>GCAGCAGC[2x]

We have analyzed crystal structures of RNA containing CAG repeats in complex with synthetic cyclic mismatch-binding ligands (CMBLs). In total, three X-ray structures consisting of (GCAGCAGC)2-CMBL3a, one structure of (GCAGCAGC)2-CMBL3b and one (GCAGCAGC)2-CMBL4 complex have been analyzed. The models show well-defined interactions between the molecules in which the CMBLs mimic nucleobases as they form pseudo-canonical base pairs with adenosine residues and engage in extensive stacking interactions with neighboring nucleotides. The binding of ligands is associated with major structural changes of the CAG repeats, which is consistent with results of biochemical studies.

The longer linker contains two N-acyl-amino groups and additional constituents: in CMBL3a it is a E-alkene, in CMBL3b it is an Z-alkene, and in CMBL4 it is an aminoalkyl moiety. One type of interaction includes the typical Watson–Crick pairing and formation of G–C and C–G pairs, which can either fill the voids between duplexes (as in seleno modified CAG(Se)-CMBL3a model) or form short insertions in the pseudo-infinite helical stack (CAG-CMBL4). In the presence of CMBL3a, the duplex is the most stable, having a melting temperature TM nearly 20°C higher. The X-ray structures show that all three ligands interact with the RNA in very similar manners, but the conformation of the bound CMBL3a is the least distorted from the idealized geometry. The asymmetric trans conformation of the long linker makes the ligand better adjusted to the binding site than the symmetric CMBL3b and CMBL4. This is consistent with the thermal melting observations that CMBL3a forms more stable complexes with the RNA than CMBL3b or CMBL4.> GPLGSPLT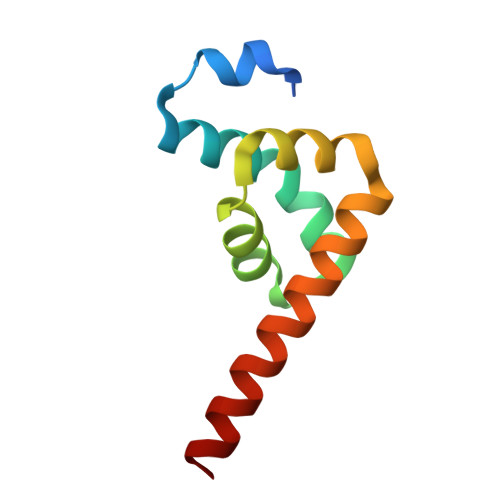ASMLASAPPQEQKQMLGERLFPLIQAMHPTLAGKITGMLLEIDNSELLHMLESPESLRSKVDEAVAVLQAHQAKEAAQKA>[12x]MEKREAQVARETGETKIEVRLSLDGT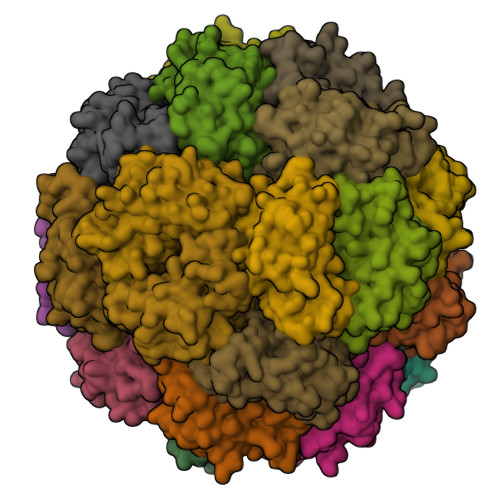GVSDVKTGIGFLDHMLSALAKHGRFDLYLRCAGDLHVDDHHTSEDCAIVLGQAFRQAIGERKGIKRYGSAYAPLDESLARAVVDISSRPFAVIDLKLKREKIGELSCEMIPHVLHSFATSANLTLHVEVLYGANDHHKAESAFKATALALREAVTKDGPADAVPSTKGVLE>GGRDKDHLLKYNVGDLVWSKVSGYPWWPCMVSADPLL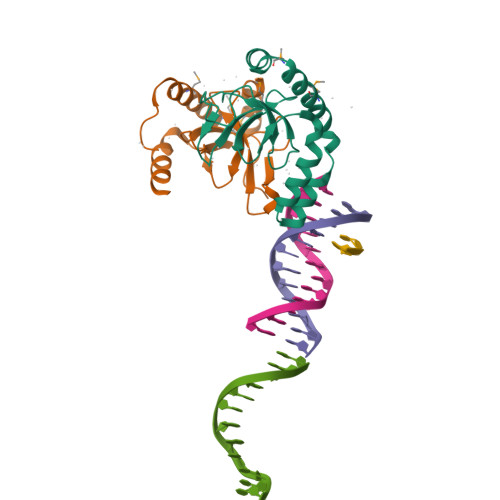HSYTKLKGQKKSARQYHVQFFGDAPERAWIFEKSLVAFEGEGQFEKLCQESAKQAPTKAEKIKLLKPISGKLRAQWEMGIVQAEEAASMSVEERKAKFTFLYVG[2x]> MASMTGGQQMGRDLQVTLYGTIKAGVEVSRVKDAGTYKAQGGKSKTATQIADFGSKIGFKGQEDLGNGMKAIWQLEQKASIAGTNSGWGNRQSFIGLKGGFGTVRAGNLNTVLKDSKDNVNAWESGSNTEDVLGLGTIGRVESREISVRYDSPVFAGFSGSVQYVPRDNANDVDKYKHTKSSRESYHAGLKYENAGFFGQYAGSFAKYADLNTDAERVAVNTANAHPVKDYQVHRVVAGYDANDLYVSVAGQYEAAKNNEVGSIKGKKHEQTQVAATAAYRFGNVTPRVSYAHGFKAKVNGVKDANYQYDQVIVGADYDFSKRTSALVSAGWLKQGKGAGKVEQTASMVGLRHKF

PorB is a trimeric anion-selective porin and the second most abundant protein in the outer membrane of N. meningitidis, possessing a binding site for antibiotics in its pore. It plays an important role in the human immune response to neisserial infections and has also been linked to inducing apoptosis upon infection of host cells. Isolates of Neisseriae with intermediate resistance to antibiotics have been reported to exhibit single-point mutations in PorB. These mutations are located in the eyelet of the pore, the narrowest region within the channels, which contains a large number of charged amino acids acting as an electrostatic filter. In this work, we show that a single point mutation in the porin PorB from Neisseria meningitidis, the causative agent of bacterial meningitis, can strongly affect the binding and permeation of beta-lactam antibiotics.

Crystals of G103K PorB from N. meningitidis W135 were grown under Jeffamine M-600 based conditions as previously reported. As a result of manual model building and interactive refinement, G103K PorB has a final Rwork/Rfree value of 21.3%/26.0% for data refined to 2.76 Å. The G103K single point mutation, located at the periplasmic side of loop L3, causes no significant changes in the secondary structure. The high degree of similarity between the G103K and wt PorB structures is reflected in a Cα root-mean-square deviation (RMSD) value of 0.278 Å (for 340 residues) (shown in Fig. 1B/C). Looking more closely at the mutation site, the loop L3 folds back from the extracellular side into the pore, forming an α-helix that constricts the pore to its narrowest point. The electron density around K103 was solved clearly from the α- to the δ‑carbon atom, whereas the density of its positively charged ε-amino group could not be determined due to the potentially high mobility of the side chain. The bulkier side chain protrudes into the pore and decreases the open cross-section of the pore constriction, approximately by 3–5 Å as compared to wt, altering the PorB filter geometry. In accordance with previous computational studies, wt PorB shows two distinct pathways for the transfer of anions and cations. In the G103K variant, the bulkier and positively charged lysine sidechain extends into the pore, thereby occupying the pathway for cations and leading to its disruption. Our experimental and computational electrophysiological data demonstrate that the conductance of G103K PorB is lower than that of the wt protein. Ampicillin transport is substantially reduced for the mutant compared to wt PorB in these experiments, demonstrating the effect of the single mutation on overall antibiotic uptake.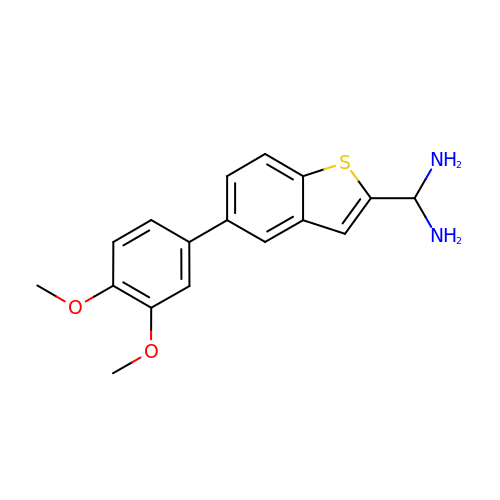1-[5-(3,4-dimethoxyphenyl)-1-benzothiophen-2-yl]methanediamine | C17 H18 N2 O2 S | XZOIHOQTJVDJCE-UHFFFAOYSA-N> MQTVGVHSIVQQLHRNSIQFTDGYEVKEDIGVGSYSVCKRCIHKATNMEFAVKIIDKSKRDPTEEIEILLRYGQHPNIITLKDVYDDGKYVYVVTELMKGGELLDKILRQKFFSEREASAVLFTITKTVEYLHAQGVVHRDLKPSNILYVDESGNPESIRICDFGFAKQLRAENGLLMTPCYTANFVAPEVLERQGYDAACDIWSLGVLLYTMLTGYTPFANGPDDTPEEILARIGSGKFSLSGGYWNSVSDTAKDLVSKMLHVDPHQRLTAALVLRHPWIVHWDQLPQYQLNRQDAPHLVKGAMAATY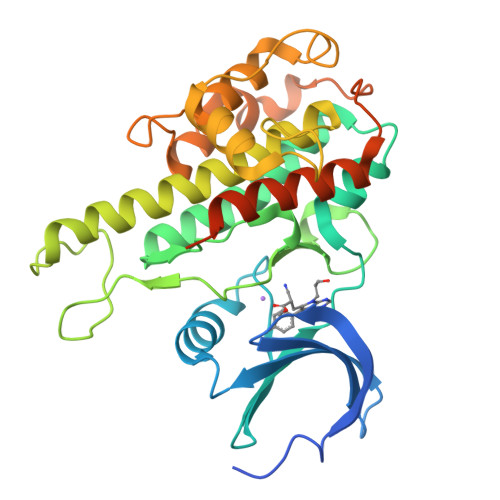SALNRNQSPVLEPVGRSTLAQRRGIKKITSTAL> MAHHHHHHMPSRRERANAIRALSMDAVQKANSGHPGAPMGMADIAEVLWRDYMQHNPSNPQWANRDRFVLSNGHGSMLIYSLLHLTGYDLGIEDLKNFRQLNSRTPGHPEYGYTAGVETTTGPLGQGIANAVGMALAEKVLAAQFNRDGHAVVDHYTYAFLGDGCMMEGISHEVASLAGTLRLNKLIAFYDDNGISIDGEVHGWFTDDTPKRFEAYGWQVIRNVDGHDADEIKTAIDTARKSDQPTLICCKTVIGFGSPNKQGKEECHGAPLGADEIAATRAALGWEHAPFEIPAQIYAEW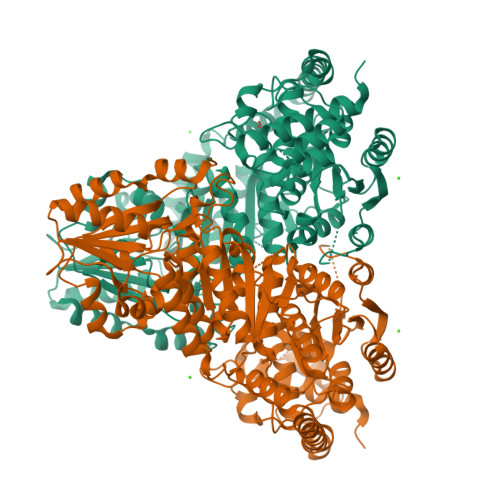DAKETGAAQEAEWNKRFAAYQAAHPELAAELLRRLKGELPADFAEKAAAYVADVANKGETIASRKASQNALNAFGPLLPELLGGSADLAGSNLTLWKGCKGVSADDAAGNYVFYGVREFGMSAIMNGVALHGGFIPYGATFLIFMEYARNAVRMSALMKQRVLYVFTHDSIGLGEDGPTHQPIEQLASLRLTPNLDTWRPADAVESAVAWKHAIERADGPSALIFSRQNLPHQARDVAQVADIARGGYVLKDCEGEPELILIATGSEVGLAVQAYDKLSEQGRKVRVVSMPCTSVYEQQDESYKQSVLPVEVGARIAIEAAHADYWYKYVGLDGRIIGMTSFGESAPAPALFEHFGFTLDNVLAVAEELLED> QVKPFSFVRDTDPVQLVNFLQSEHPQTIAVVLSYLDPPVAAQILGALPEELQTEVLKRIALLERTSVKEIERNLEKKISGFVSRTFSKVGGIDTAAEIMNNLDRTTEKKIMDKLVQENPELADEIRRRMFVFEDILKLDDRSIQLVLREVDTRDLALALKGASDELKEKIFKNMSKRAAALLKDELEYMGPV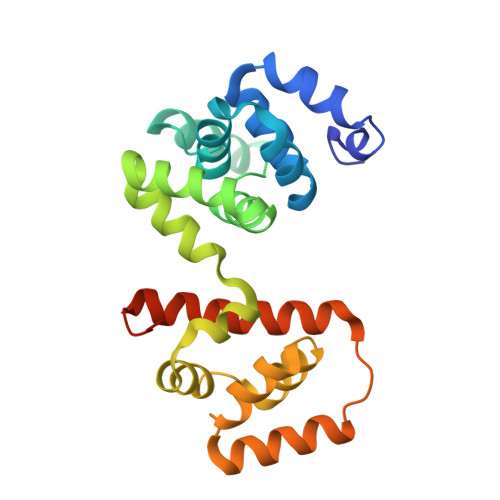RLKDVEEAQQKIINIIRRLEEAGEIVIARGGGEELIM D-glycero-alpha-D-manno-heptopyranose 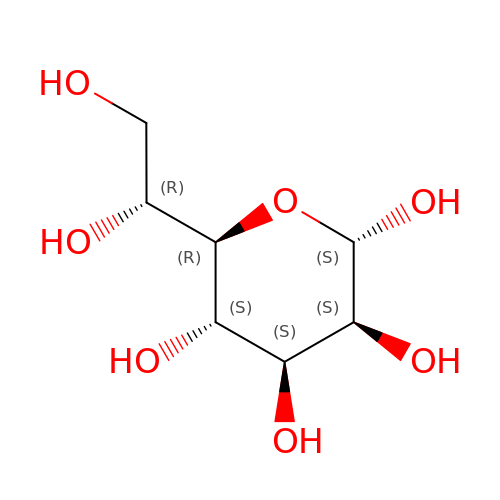| C7 H14 O7 | BGWQRWREUZVRGI-QTNLNCNHSA-N> AIQ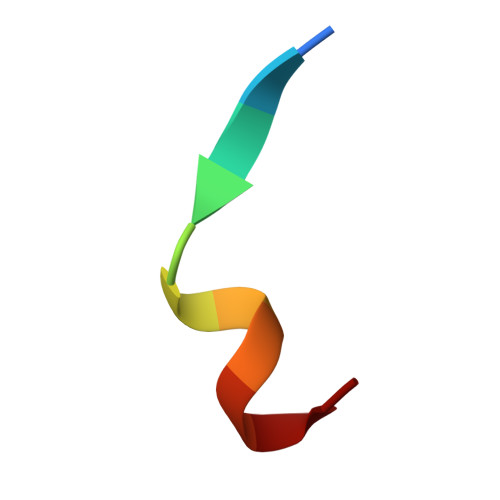SEKARKHN> GPLGSMNRVEAARNVHIVGSGDTTVVLGHGFGTDQSVWKHLVPYLVDSYRVLLYDNMGAGSTNPEYFHFERYSTLQGYAHDLLVILHEFNIRSCIFVGHSLSAMTGAIASIIRPDLFQKIVMLSASPRFLNTADYLGGFEPADVEQLAGAIEANYKSWVSGF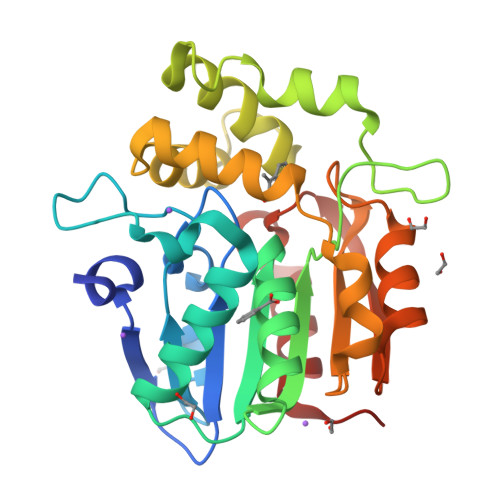APMVVGGDMDSVAVQEFSRTLFNMRPDIARSVFRTIFTSDLRDYLGRVTVPCHIIQSSRDMAVPVSVAGYIHNRVGGRSVVEVMNTEGHLPQLSAPEVAIPVLLRHIKNDIDS>GGVEVLEVKTGVDAITEVECFLNPEMGDPDENLRGFSLNLSAENDFSSDSPQRKMLPCYSTARIPLPNLNEDLTSGNLLMWEAVTVQTEVIGITSMLNLHAGSQKVHEHGGGKPIQGSNFHFFAVGGEPLEMQGVLMNYRSKYPDGTITPKNPTAQSQVMNTDHKAYLDKNNAYPVECWVPDPSRNENARYFGTFTGGENVPPVLHVTNTATTVLLDEQGVGPLCKADSLYVSAADICGLFTNSSGTQQWRGLARYFKIRLRKRSVKNPYP[10x]

BK polyomavirus (BKPyV) is a small, non-enveloped, double-stranded DNA virus with an icosahedral capsid formed by 72 capsomers, where a capsomer is an association of a pentamer of the VP1 protein linked internally to a single copy of either the VP2 or the VP3 proteins. BK polyomavirus (BKPyV) is an opportunistic pathogen that uses the b-series gangliosides GD1b and GT1b as entry receptors. Viruses sampled sequentially from these patients accumulated multiple mutations in the BC loop region of the VP1 protein, which is involved in the direct interaction of the virus with sialic acids. All variant VP1 pentamer structures were globally similar to the WT VP1 pentamer with a doughnut-shaped ring composed of a central pore surrounded by five VP1 monomers in 5-fold symmetry.

The structure of the N-Q variant VP1 pentamer was also solved at 2.01 Å. Although no major change was observed in the backbone orientation of the BC loop that carried the K69N and E82Q mutations, the mutation from lysine to asparagine at position 69 modified the sialic acid binding pocket of the VP1 pentamer. Lysine 69 is involved directly with the double sialic acid part of the b-series gangliosides by making van der Waals, salt bridge, and hydrogen bond interactions through its side chain, and its replacement by asparagine leads to loss of those interactions. On the other hand, the K69N mutation in the K69N-E82Q variant leads to a steric clash that precludes sialic acid binding. Here also with the double mutant VP1, N-Q, in sharp contrast to the other four VP1 proteins, binding was not detected to any sialylated or non-sialylated glycans included in the screening arrays. Also consistent with the glycan array results, N-Q VLPs did not bind any of the tested gangliosides. However, the N-Q variant maintained its ability to infect 293TT cells after sialic acid removal, indicating that its infection occurs in a sialic acid-independent manner. Thus, another receptor must be involved to support N-Q variant infection in 293TT cells. Finally, as predicted, no infection was seen in any supplementation condition for the N-Q variant, confirming that gangliosides are not used by this variant for infectious entry. The N-Q variant lost binding to sialylated glycans, but it retained some infectivity, suggesting that in certain conditions, BKPyV may interact directly with the unknown receptor for entry.> MGSSHHHHHHSSGRENLYFQGHMNGDQNSDVYAQEKQDFVQHFSQIVRVLTEDEMGHPEIGDAIARLKEVLEYNAIGGKYNRGLTVVVAFRELVEPRKQDADSLQRAWTVGWCVELLQAFFLVADDIMDSSLTRRGQICWYQKPG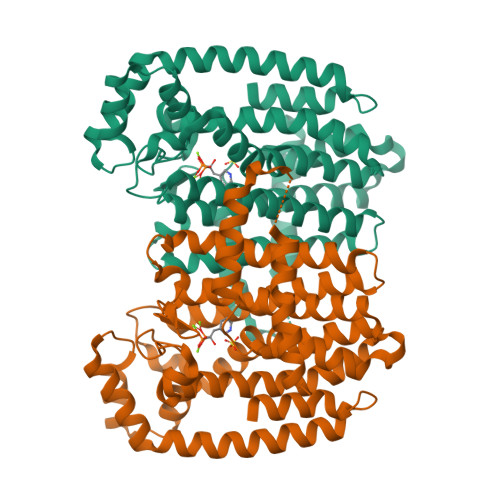VGLDAINDANLLEACIYRLLKLYCREQPYYLNLIELFLQSSYQTEIGQTLDLLTAPQGNVDLVRFTEKRYKSIVKYKAAFYSFYLPIAAAMYMAGIDGEKEHANAKKILLEMGEFFQIQDDYLDLFGDPSVTGKIGTDIQDNKCSWLVVQCLQRATPEQYQILKENYGQKEAEKVARVKALYEELDLPAVFLQYEEDSYSHIMALIEQYAAPLPPAVFLGLARKIYKRRK>[4x]GSHMEAVQNRIVEAAERVPGVRGVIHLRARYVGQDIWAD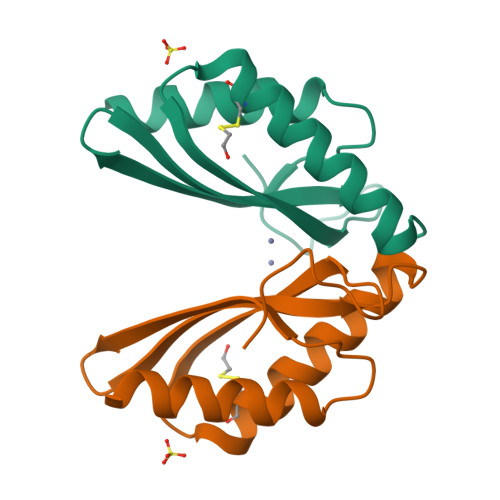MIIGVDPENTVEQAEEICEAVQAAVCGKIRRIESLHVSAEAREIGDTTKPSFSDQPLSFDEVMLSKVDN[METHYLSELENO]ACETATE | C3 H5 O2 Se | 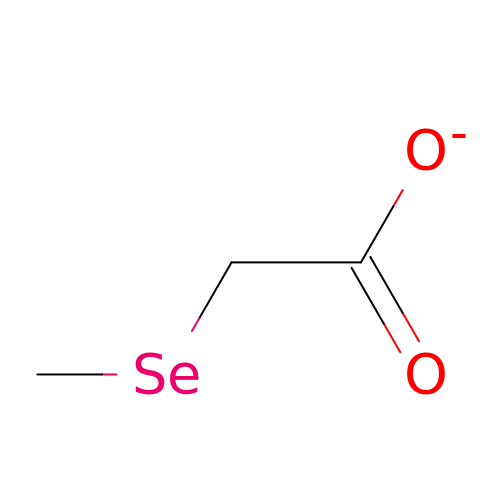UOULLTHLSZQUIN-UHFFFAOYSA-M>MRVLALSAVFLVASIIGMPAVAKEWQENKSWNAHFTEHKSQGVVVLWNENKQQGFTNNLKRANQAFFPASTFKIPNSLIALDLGVVKDEHQVFKWDGQTRDIATWNRDHNLITAMKYSVVPVYQEFARQIGEARMSKMLHAFDYGNEDISGNVDSFWLDGGIRISATEQISFLRKLYHNKLHVSERSQRIVKQAMLTEANGDYIIRAKTGYSTRIEPKIGWWVGWVELDDNVWFFAMNMDMPTSDGLGLRQAITKEVLKQEKIIP[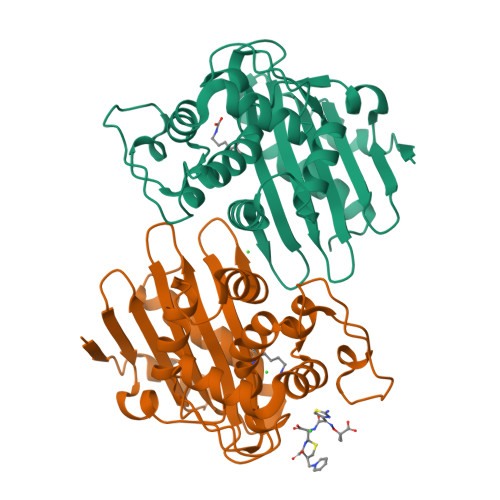4x]We have focused our work on the iron(II)/α-KetoAcid-dependent Oxygenases (αKAOs), a mechanistically diverse superfamily of enzymes that use dioxygen as the oxidant to catalyze several reactions via C-H bond activation, mostly hydroxylation. These enzymes operate with three substrates, dioxygen, α-ketoglutarate (α-KG) and a primary substrate. One of these, KDO1, catalyzes the formation of (3S)-3-hydroxy-L-lysine, while five others, KDO2 to KDO6, promote the formation of (4R)-4-hydroxy-L-lysine. We based our analysis on the structures that we solved by X-ray crystallography of two of the regiodivergent αKAOs active towards L-lysine, namely KDO1 from Catenulispora acidiphila, that catalyzes the C-3 hydroxylation, and KDO5, from Flavobacterium sp., that catalyzes the C-4 hydroxylation.

The structure of the apo form of KDO1 was determined without iron in the active site, lost during purification, while KDO5 retained the iron throughout. While a ferrous ion is present in the KDO5 apo structure, it is not the case in KDO1 apo as the metal is lost during the purification from the KDO1 preparation used to grow the crystals. In all four molecules of each of the KDO5 structures, an iron ion is present in the active site chelated by two His (176 and 312) and one Glu (178). In KDO5 the pocket is characterized by a neck defined by four residues, namely, Trp112, Arg145, Asn232 and Asp230. Of these, Arg145 is instrumental in the recognition of L-lysine, as it is able to attract the substrate towards the end of the pocket where it can be maintained during the reaction.

>[4x]MKSQSIMSVERSAETSLTLEIPTSPLIIKITQQERNILSNVGNLLVKAFGNYENPDYIASLHLHAFQLLPERITRILSQFGSDFSAEQYGAIVFQGLIEVDQDDLGPTPPNWQGADYGKLNKYGFICSLLHGAVPSKPVQYYAQRKGGGLLHAVIPDEKMAATQTGSGSKTDLFVHTEDAFLSNQADFLSFLYLRNEERVPSTLYSIRSHGKMNPVMKKLFEPIYQCPKDANYNDEDVANSGPTASVLYGNRELPFIRFDAAEQIFNENAGQTSEALGNLMDFWDEAKTLINSDYIPNSGDLIFVNNHLCAHGRSAFIAGQRIENGEIIKCERRQMLRMMSKTSLIHIRSVTRTDDPYFIMEEHLGKIFDLD>[2x]MALRVAAFDLDGVLALPSIAGAFRRSEEALALPRDFLLGAYQTEFPEGPTEQLMKGKITFSQWVPLMDESYRKSSKACGANLPENFSISQIFSQAMAARSINRPMLQAAIALKKKGFTTCIVTNNWLDDGDKRDSLAQMMCELSQHFDFLIESCQVGMIKPEPQIYNFLLDTLKAKPNEVVFLDDFGSNLKPARDMGMVTILVHNTASALRELEKVTGTQFPEAPLPVPCNPNDVS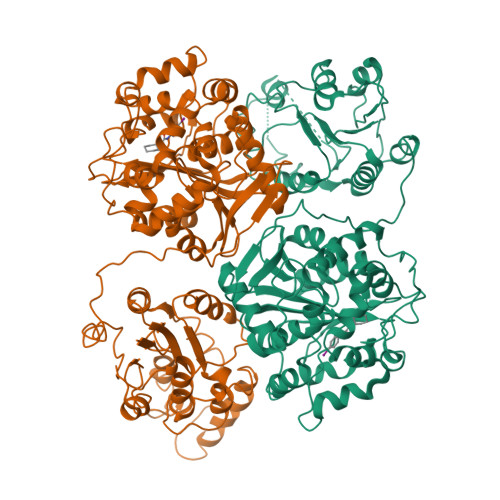HGYVTVKPGIRLHFVEMGSGPALCLCHGFPESWFSWRYQIPALAQAGFRVLAIDMKGYGDSSSPPEIEEYAMELLCKEMVTFLDKLGIPQAVFIGHDWAGVMVWNMALFYPERVRAVASLNTPFMPPDPDVSPMKVIRSIPVFNYQLYFQEPGVAEAELEKNMSRTFKSFFRASDETGFIAVHKATEIGGILVNTPEDPNLSKITTEEEIEFYIQQFKKTGFRGPLNWYRNTERNWKWSCKGLGRKILVPALMVTAEKDIVLRPEMSKNMEKWIPFLKRGHIEDCGHWTQIEKPTEVNQILIKWLQTEVQNPSVTSKI3,4-DIMETHYLTHIAZOLIUM ION | C5 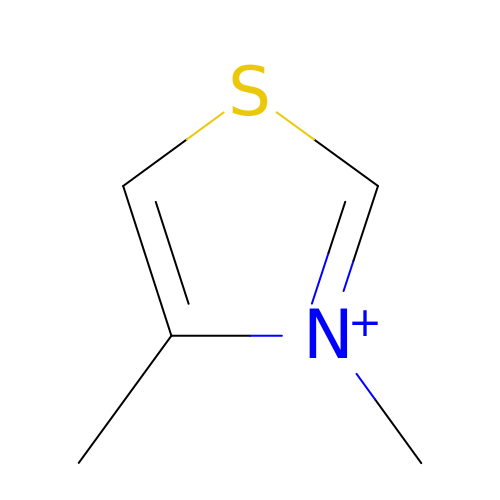H8 N S | RHRPPNDIWVFSRX-UHFFFAOYSA-N> MKVTIIGASGRVGSATALLLAKEPFMKDLVLIGREHSINKLEGLREDIYDALAGTRSDANIYVESDENLRIIDESDVVIITSGVPRKEGMSRMDLAKTNAKIVGKYAKKIAEICDTKIFVITNPVDVMTYKALVDSKFERNQVFGL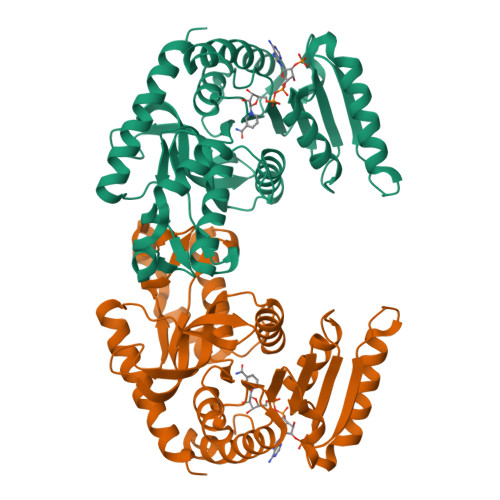GTHLDSLRFKVAIAKFFGVHIDEVRTRIIGEHGDSMVPLLSATSIGGIPIQKFERFKELPIDEIIEDVKTKGEQIIRLKGGSEFGPAAAILNVVRCIVNNEKRLLTLSAYVDGEFDGIRDVCIGVPVKIGRDGIEEVVSIELDKDEIIAFRKSAEIIKKYCEEVKNL MBH reactions are valuable carbon-carbon bond forming transformations in organic synthesis, for which no natural enzymes are known. Previous work has afforded the MBHase BH32.1413 which promotes catalysis via a histidine nucleophile. In this work, His23 is replaced by Nδ-methylhistidine (MeHis) for the creation of a more efficient MBHase. In this study, we explore the evolutionary trajectory of a BH32 variant with MeHis in place of His23.

To identify a suitable starting template for engineering a MeHis-containing MBHase, we replaced the His23 nucleophile of BH32 and selected evolved descendants with MeHis using an engineered pyrrolysyl-tRNA synthetase/tRNA pair. In contrast to the improved hydrolytic activity observed upon His23MeHis substitution in BH3220, MBH activity was reduced upon MeHis incorporation across all BH32 variants. Of the modified variants tested, BH32.8 His23MeHis (subsequently referred to as BHMeHis1.0) was found to have the highest activity and was selected for further engineering. BHMeHis1.0 was also found to have an altered pH optimum compared to BH32.8, with the highest conversion observed at pH 6.0. To gain insights into this mechanism, crystal structures of apo-BHMeHis1.0 and apo-BHMeHis1.8 were solved. Efforts to obtain structures complexed with either substrate(s) or product have thus far been unsuccessful. Comparison of the BHMeHis1.8 and BHMeHis1.0 structures reveals that the 23 mutations installed during evolution cause minimal changes to the overall protein fold (secondary structure root mean square deviation (rmsd) 0.47 Å, Supplementary Fig. 9). The MeHis nucleophile adopts a single conformation in the structures of BHMeHis1.8 and BHMeHis1.0, however a notable 120° rotation of the imidazole ring has occurred. The first four mutations introduced into BHMeHis1.0 during rounds 1 and 2 of evolution gave a > 4-fold increase in activity. In contrast, these mutations reduce activity in the analogous His23 containing variant (BH32.8), and therefore would not have been selected if evolving with His23 as the catalytic nucleophile.

> MIRAVFFDSLGTLISVEGAYKVHLKIMEEVLGDYPLNPKTLLDEYEKLAREAFSNYAGKPYRPLRDILEEVMRKLAEKYGFKYPENLWEISLRMAQRYGELYPEVVEVLKSLKGKYHVGVILNRDTEPATAFLDALGIKDLFDSITTSEEAGFFKPHPRIFELALKKAGVKGEKAVYVGDNPVKDAGGSKNLGMTSILLDRKGEKREFWDKADFIVSDLREVIKIVDELNGQGSLEHHHHHH> ASSPANKVYQDRFESMYSKIKDPANGYFSEQGIPYHSIETLMVEAPDYGHVTTSEAMSYYMWLEAMHGRFSGDFTGFDKSWSVTEQYLIPTEKDQPNTSMSRYDANKPATYAPEFQDPSKYPSPLDTSQPVGRDPINSQLTSAYGTSMLYGMHWILDVDNWYGFGARADGTSKPSYINTFQRGEQESTWETIPQPCWDEHKFGGQYGFLDLFTKDTGTPAKQFKYTNAPDADARAVQATYWADQWAKEQGKSVSTSVGKAT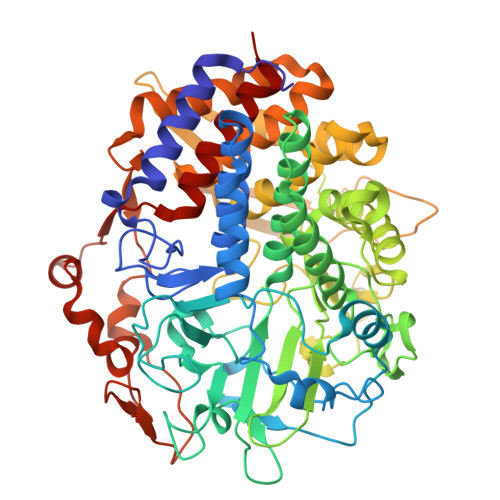KMGDYLRYSFFDKYFRKIGQPSQAGTGYDAAHYLLSWYYAWGGGIDSTWSWIIGSSHNHFGYQNPFAAWVLSTDANFKPKSSNGASDWAKSLDRQLEFYQWLQSAEGAIAGGATNSWNGRYEAVPSGTSTFYGMGYVENPVYADPGSNTWFGMQVWSMQRVAELYYKTGDARAKKLLDKWAKWINGEIKFNADGTFQIPSTIDWEGQPDTWNPTQGYTGNANLHVKVVNYGTDLGCASSLANTLTYYAAKSGDETSRQNAQKLLDAMWNNYSDSKGISTVEQRGDYHRFLDQEVFVPAGWTGKMPNGDVIKSGVKFIDIRSKYKQDPEWQTMVAALQAGQVPTQRLHRFWAQSEFAVANGVYAILFPD> DVSFRLSGADPRSYGMFIKDLRNALPFREKVYNIPLLLPSVSGAGRYLLMHLFNYDGKTITVALDVTNVYIMGYLADTTSYFFNEPAAELASQYVFRDARRKITLPYSGNYERLQIAAGKPREKIPIGLPALDSAISTLLHYDSTAAAGALLVLIQTTAEAARFKYIEQQIQERAYRDEVPSLATISLENSWSGLSKQIQLAQGNNGIFRTPIVLVDNKGNRVQITNV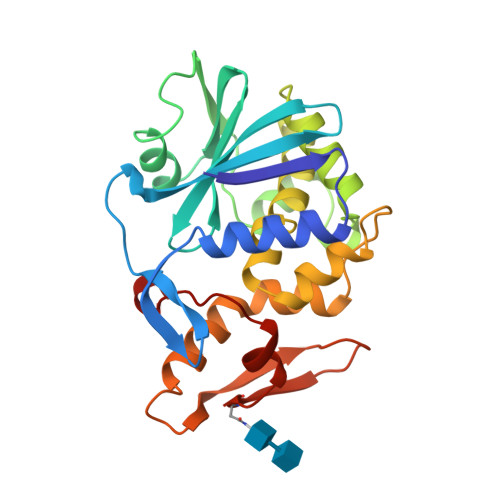TSKVVTSNIQLLLNTRNI Na+–K+–Cl− cotransporters functions as an anion importers, regulating trans-epithelial chloride secretion, cell volume, and renal salt reabsorption. Loop diuretics, including furosemide, bumetanide, and torsemide, antagonize both NKCC1 and NKCC2, and are first-line medicines for the treatment of edema and hypertension. Here we determined three cryo-EM structures of phosphorylated NKCC1 individually bound with furosemide, torsemide, and bumetanide, unlocking two modes of interaction of loop diuretics with NKCC1. In all the three co-structures, NKCC1 assembled as a C2-symmetric dimer in which two TMDs are separated by ~30 Å within the lipid bilayer and two cytosolic C-terminal domains (CTDs) interdigitate and associate extensively with the TMDs from beneath.

Torsemide lacks the carboxyl group which is indispensable for furosemide and bumetanide to co-occlude a K+ ion and contributes to their K+-dependent antagonism on NKCCs. Our NKCC1/torsemide co-structure showed that torsemide adopts a U-shape configuration with its sulfonylpyridine group, which marks the U-turn, facing TM1b and TM6a on one side and the propan-2-ylurea and methylanilino groups projecting toward TM3 and TM8 on the other side (D and EV3C). Torsemide notably reaches slightly deeper into the NKCC1 ion translocation path than do furosemide and bumetanide, and in doing so, it completely occupies and expels ions from the Cl− site 1 and K+ site. Just beneath the extracellular ion entryway, torsemide’s propan-2-ylurea group forms salt bridge with the main chain nitrogen atom of Val302 in TM1a and also engages with Gly301, Val302, and Met303 in TM1a and Met382 in TM3 via hydrophobic interactions. At the U-turn, torsemide’s sulfonylpyridine group establishes hydrophobic interactions with Ala497 and Pro496 in the TM6b. Further toward the midway of NKCC1 ion translocation path, torsemide’s methylanilino group projects toward a hydrophobic pocket and interacts with Tyr383 in TM3, and Ile677 and Ser678 in TM8. Our MD results showed that the favored (i.e., more stable) state of torsemide is the one that features a protonated and positively charged pyridine (Tor_NH_N, Fig. EV4E–G). In this state, torsemide’s pyridine can replace the K+ ion in its binding site, while its deprotonated and negatively charged sulfonylurea can substitute the Cl− ion at the so-called site 1. On the other hand, torsemide encroaches into and expels the K+ ion from its binding site, suggesting that it could be more potent under low [K+] conditions. Another intriguing finding regarding loop diuretic pharmacology is that the sulfamoyl group of furosemide and bumetanide directly engages with extracellular gate residues of NKCC1, but torsemide’s sulfamoyl group reaches further toward the midway point of the ion translocation path and makes no obvious contact with NKCC1.

>[2x]MEPRPTAPSSGAPGLAGVGETPSAAALAAARVELPGTAVPSVPEDAAPASRDGGGVRDEGPAAAGDGLGRPLGPTPSQSRFQVDLVSENAGRAAAAAAAAAAAAAAAGAGAGAKQTPADGEASGESEPAKGSEEAKGRFRVNFVDPAASSSAEDSLSDAAGVGVDGPNVSFQNGGDTVLSEGSSLHSGGGGGSGHHQHYYYDTHTNTYYLRTFGHNTMDAVPRIDHYRHTAAQLGEKLLRPSLAELHDELEKEPFEDGFANGEESTPTRDAVVTYTAESKGVVKFGWIKGVLVRCMLNIWGVMLFIRLSWIVGQAGIGLSVLVIMMATVVTTITGLSTSAIATNGFVRGGGAYYLISRSLGPEFGGAIGLIFAFANAVAVAMYVVGFAETVVELLKEHSILMIDEINDIRIIGAITVVILLGISVAGMEWEAKAQIVLLVILLLAIGDFVIGTFIPLESKKPKGFFGYKSEIFNENFGPDFREEETFFSVFAIFFPAATGILAGANISGDLADPQSAIPKGTLLAILITTLVYVGIAVSVGSCVVRDATGNVNDTIVTELTNCTSAACKLNFDFSSCESSPCSYGLMNNFQVMSMVSGFTPLISAGIFSATLSSALASLVSAPKIFQALCKDNIYPAFQMFAKGYGKNNEPLRGYILTFLIALGFILIAELNVIAPIISNFFLASYALINFSVFHASLAKSPGWRPAFKYYNMWISLLGAILCCIVMFVINWWAALLTYVIVLGLYIYVTYKKPDVNWGSSTQALTYLNALQHSIRLSGVEDHVKNFRPQCLVMTGAPNSRPALLHLVHDFTKNVGLMICGHVHMGPRRQAMKEMSIDQAKYQRWLIKNKMKAFYAPVHADDLREGAQYLMQAAGLGRMKPNTLVLGFKKDWLQADMRDVDMYINLFHDAFDIQYGVVVIRLKEGLDISHLQGQEELLSSQEKSPGTKDVVVSVEYSKKSDLDTSKPLSEKPITHKVEEEDGKTATQPLLKKESKGPIVPLNVADQKLLEASTQFQKKQGKNTIDVWWLFDDGGLTLLIPYLLTTKKKWKDCKIRVFIGGKINRIDHDRRAMATLLSKFRIDFSDIMVLGDINTKPKKENIIAFEEIIEPYRLHEDDKEQDIADKMKEDEPWRITDNELELYKTKTYRQIRLNELLKEHSSTANIIVMSLPVARKGAVSSALYMAWLEALSKDLPPILLVRGNHQSVLTFYS ISOPENTYL PYROPHOSPHATE | C5 H14 O7 P2 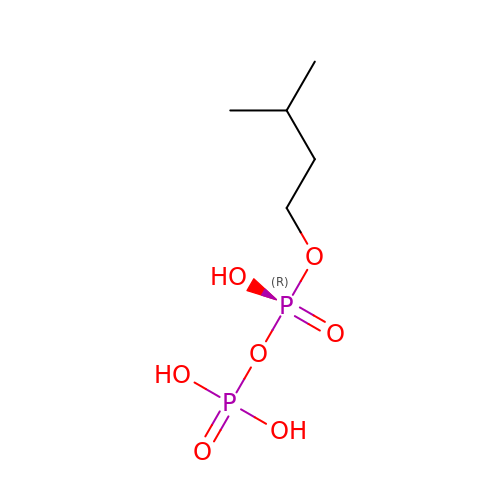| IPFXNYPSBSIFOB-UHFFFAOYSA-N> MHHHHHH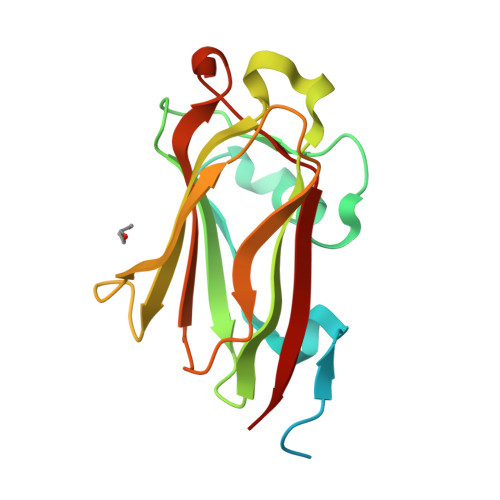SSGRENLYFQGFCGRSGKQLKRCHSSQPGMLLDSWSRMVKSLNVSSSVNQASRLIDGSEPCWQSSGSQGKHWIRLEIFPDVLVHRLKMIVDPADSSYMPSLVVVSGGNSLNNLIELKTININPSDTTVPLLNDCTEYHRYIEIAIKQCRSSGIDCKIHGLILLGRIR>MMMASKDAPSNMDGTSGAGQLVPEVNAAEPLPLEPVVGAATAAATAGQVNLIDPWIMNNFVQAPEGEFTISPNNTPGDILFDLHLGPHLNPFLQHLSQMYNGWVGNMRVRVMLAGNAFTAGKIIICCVPPGFASQNISIGQATMFPHVIADVRVLEPIEIPLDDVRNVLFHTNENRPTMRLLCMLYTPLRAGGASSGTDPFVIAGRVLTCPSPDFNFLFLVPPSVEQKTRQLTVPNIPLNNLANSRVPAMINKMTVSTDQNQVVQFQ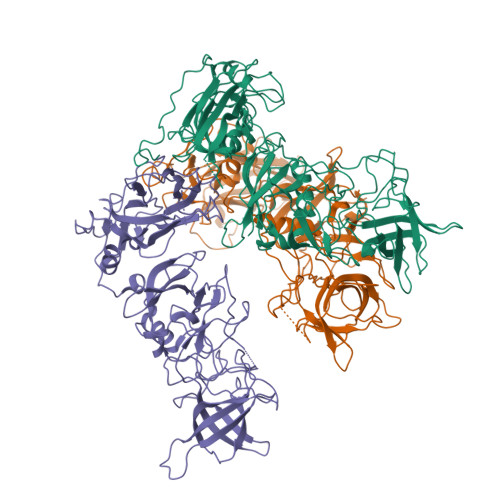NGRCTLEGQLLGTTPVSASQVARIRGKVFSTASGKGLNLTELDGTPYHAFESPAPLGFPDIGACDWHVSTFKVDQNLSGDPMSRLDVKQNAPFAPHLGSIEFTSDQDPTGDQLGTLAWVSPSTSGARVDPWKIPSYGSTVTESTHLAPPIFPPGFGEAIVYFMSDFPIVSGNTAQVPCTLPQEFVSHFVEQQAPVRGEAALLHYVDPDTHRNLGEFKLYPDGFITCVPNTGGGPQNLPTNGVFVFSSWVSRYYQLKPVGTAGPARRLGVRRV[3x]> MAVLYPQVIVDHPFFFLIRNRRTGTILFMGRV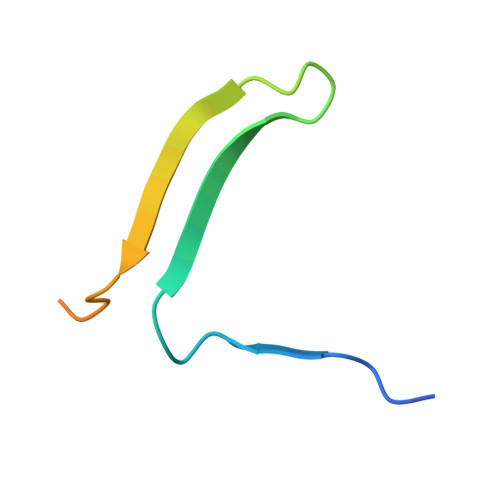MHPETMNTSGHDFEEL>ALVDVFIKLDGTGNLLVLRTLPGNAHAIGVLLDNLDWDEIVGTICGDDTCLIICRTPKDAKKVSNQLLSML[3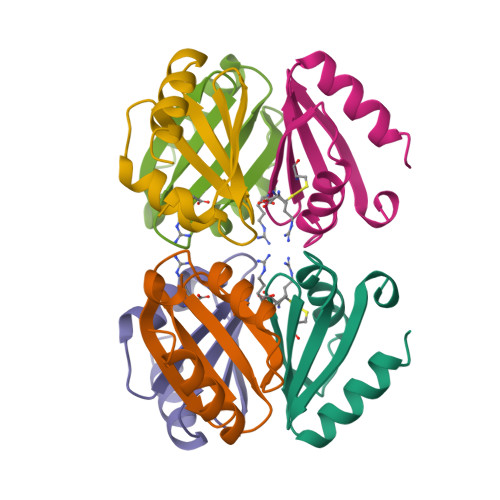x]> SHDGNSQQGSGSDGGSSMCLELALEGERLCKAGDCRAGVAFFQAAIQAGTEDLRTLSAIYSQLGNAYFYLGDYNKAMQYHKHDLTLAKSMNDRLGEAKSSGNLGNTLKVMGRFDEAAICCERHLTLARQLGDRLSEGRALYNLGNVYHAKGKHLGQRNPGKFGDDVKEALTRAVEFYQENLKLMRDLGDRGAQGRACGNLGNTYYLLGDFQAAIEHHQERLRIAREFGDRAAERRANSNLGNSHIFLGQFEDAAEHYKRTLALAVELGEREVEAQSCYSLGNTYTLLHEFNTAIEYHNRHLAIAQELGDRIGEARACWSLGNAHSAIGGHERALKYAEQHLQLAKELHDPVGEST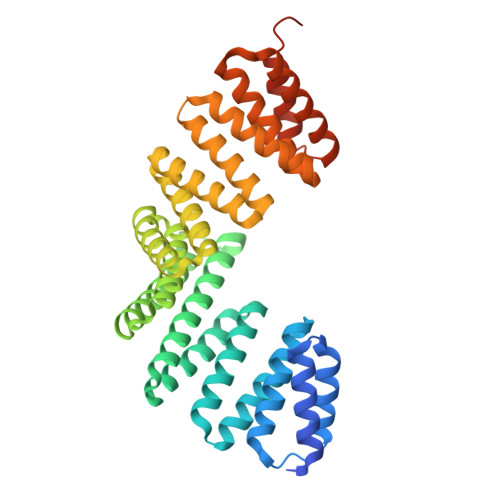ARVNISDLRKLLGMPDSEPSPTEEEAR> MVRKVFNDGDILYAEDVNIIGQPFVDGQDLLGHGLKVDDNSLSDEPQNIKTRFYAWYNRFRVTVQSGLTLSVTQGSISVSGNIISFPPQTIN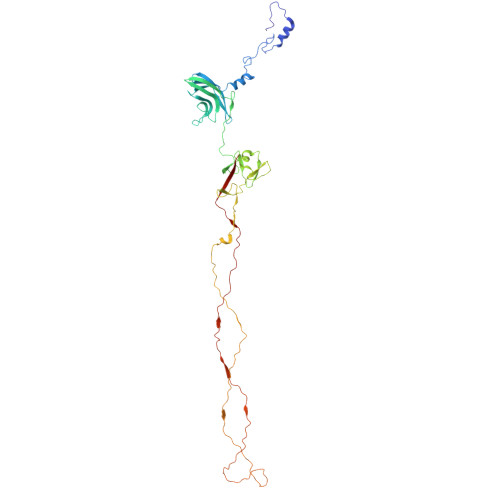AIDNANSFVWIGKTDADPAIALRVSQTLPNVCIPLARVIAASGSVTSVTDLRDVSVDILPPSIPDAVPVGSTIISLIPPTAPIPAGYLELLNSSQNVSRTTYSALFVLWGTYYGNGDGSTTFGVPGTGGRFLRLGGSGLSVGDIGGSNQITIPTNALPSHQHGIPANTHTHSVNDGGHGHTINQTPHSHSISDPGHAHGVPFGAAVDNGNNAFDTGGSPYNNGIGTTQNQTGISVNTANANLSINTSSTGISIQSASTGLTVTSNAGNGQAFQHDQPYLVFRVFVKV> STGNASDSSSDSSSSEGDGTVSSA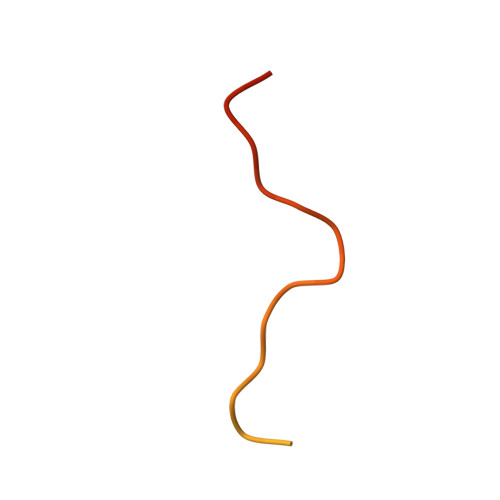DPNSDWNAPAEEWGNWVDE> MATDVAQGPNGRALAESMNPDLLSAIQQHISIERYASVTYLAMSIWCAERE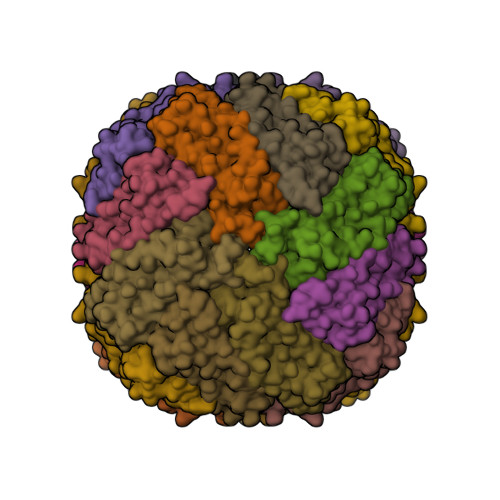LAGFYQFFDGEAKDEQSHAVHFTQYLIARSQSNDLQTLDAPRQNWDSLASLMATAFQMEADTTSSIQSVYALAERNSDTRTTVFLDPLIDAQIQSEDQFAYLLGRVKFANGDPTALLVIDNELRAGQTQRG> GACSNDEEMATGGQNQLPVDGREAYMSVSVAMPKSTGTRALGEHHGTADEQNVKEVLLALFDASDVCLETKTLATTDYILNVGGANKAGYDGKAFKVPSATAKVLAVVNPSDKFKTACVASASWSAINGAVEQTLDEVTGTSKNNFMMINAGDNANPTNGALVTANVKVVDGTTIPDVATAISEAQADRSMIYVDRVVAKVSLGTNPDGLKVPAGVTCTFGDWALNITNKSMFPYSEIVMPAGGSTGADYRIDPNYELAGFDVSQFNYLKVADDGTLPADFSAMADSKYCLENTMAADAQTQAQTTSAVASAVYTPGSFTVGESWFRLLGVTYKTLADLQVVYNAAKAAGTADAAQTQVITLCDQFYARIAKAATAQGKAVGADFASITITELDDLKSGGEYSKPDAAAGETVGVEYFQKGVCYYNILIHHDDAITATMAHGKYGVVRNNWYTLTINSVKQPGTPWLPDTTNPTDPKDP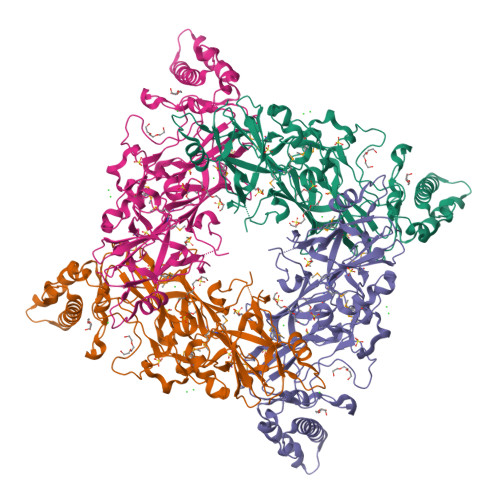GEDDDDKEAYLSVEITVNPWTTWSQGVDL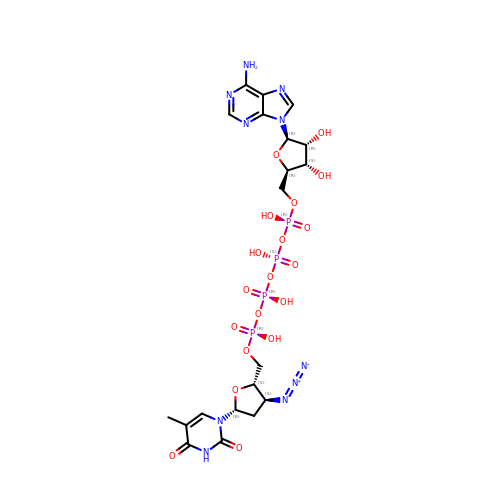[[[[(2R,3S,4R,5R)-5-(6-aminopurin-9-yl)-3,4-dihydroxy-oxolan-2-yl]methoxy-hydroxy-phosphoryl]oxy-hydroxy-phosphoryl]oxy-hydroxy-phosphoryl] [(2S,3S,5R)-3-azido-5-(5-methyl-2,4-dioxo-pyrimidin-1-yl)oxolan-2-yl]methyl hydrogen phosphate | C20 H28 N10 O19 P4 | NHJROJSMKQZWCP-SLFMBYJQSA-N>[8x]MAEVVNISKSASFSKQEKEFSDFQKSKESNEKILNKESNRFTLHPIMYPEVWNFYKKAEASFWTAEEIDLSSDLKDFE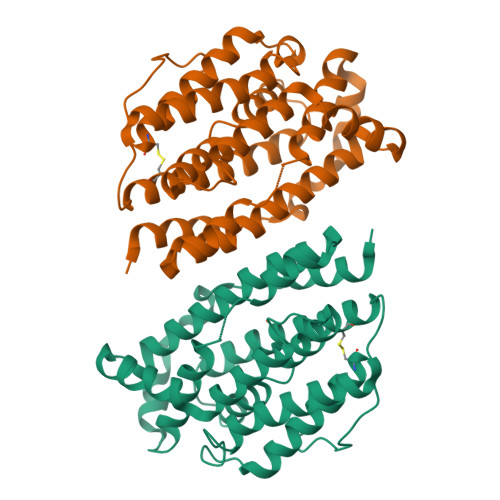KLNVNEKHFIKHVLAFFAASDGIVLENLASKFLREVEIIEAKKFYSFQIAVENIHSETYSLLIDNYIKDEKERLNLFHAIENIPAIKNKALWAAKWINDTNSFAERIVANACVEGILFSGSFCAIFWFKKQNKLHGLTFSNELISRDEGLHTDFNCLIYSLLENKLPENVVQNIVKEAVEVERSFICESLPCDLIGMNSRLMSQYIEFVADRLLECLGCSKVFHSKNPFNWMDLISLQGKTNFFEKRVADYQKSGVMAQRKEQVFSLNTDF>MKLPIHFYKPLAAGAP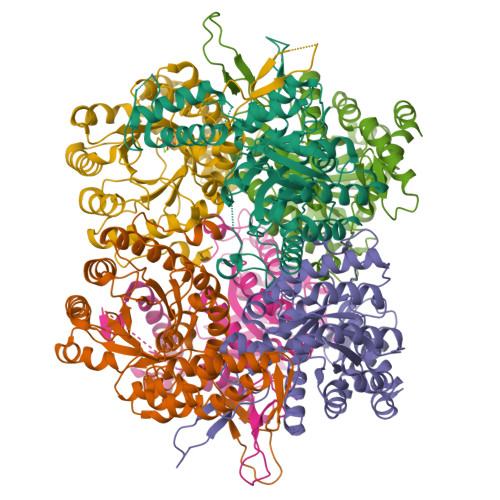QPIRELPVRPERVIHFFPPHVEKIRARIPEVAKQVDVLCGNLEDAIPIDAKEAARAGFIEVARNTDFGDTALWVRVNALNSPWVLDDIADIVATVGNKLDVMMIPKVEGPWDIHFVDQYLALLEAKHQIQKPILIHALLETAQGMMNLEAIAGASPRMHGFSLGPADLAASRGMKTTRVGGGHPFYGVLADPQEGQEHRPFYQQDLWHYTIARMVDVAVAHGLRAFYGPFGDIKDEAACEAQFRNAFLLGCTGAWSLAPNQIPIAKRVFSPDVNEVLFAKRILDAMPDGSGVAMIDGKMQDDATWKQAKVIVDLARMIAKKDPELAQAYGF[12x]> AVCPDGTRVSHAACCAFIPLAQDLQETIFQNECGEDAHEVIRLTFHDAIAISRSQGPKAGGGADGSMLLFPTVEPNFSANNGIDDSVNNLIPFMQKHNTISAADLVQFAGAVALSNCPGAPRLEFLAGRPNKTIAAVDGLIPEPQDSVTKILQRFEDAGGFTPFEVVSLLASHSVARA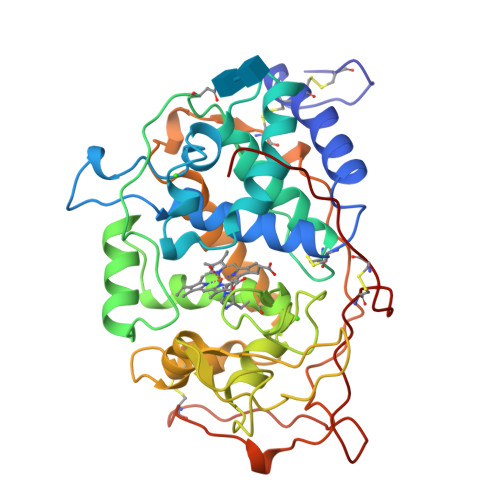NKVDQTIDAAPFDSTPFTFDTQVFLEVLLKGVGFPGSANNTGEVASPLPLGSGSDTGEMRLQSDFALAHDPRTACIWQGFVNEQAFMAASFRAAMSKLAVLGHNRNSLIDCSDVVPVPKPATGQPAMFPASTGPQDLELSCPSERFPTLTTQPGASQSLIAHCPDGSMSCPGVQFNGPA The temperate phage lambda, which infects the bacterium Escherichia coli, belongs to Siphoviridae. The virion of the lambda phage comprises an icosahedral head and a long flexible tail. The tail, which comprises the tail tube and tail tip, connects with the head through the neck. The neck–tail complex comprises a channel formed by stacked 12-fold and hexameric rings and a 3-fold symmetrical tip.

Each of the 32 rings of gpV is assembled by 6 copies of the major tail protein gpV wrapped around an oligomer of the tape measure protein gpH. The 32 rings form a right-handed helix with an axial rise of approximately 42 Å and a twist of approximately 17.5° for 2 adjacent rings. GpV has 2 distinctive domains: the N-terminal domain (gpVN, residues 3–156) and the C-terminal domain (gpVC, residues 157–246). The inner tube structure could be reconstructed to a resolution of 3.5 Å, which enabled us to build an atomic model of the gpVN domain (S1B). The gpVN domain comprises a β-sandwich flanked by an α-helix. The β-sandwich is inserted by an E-loop (residues 50–78) between β3 and β4 and by an O-loop (residues 24–38) between β1 and β2. Six copies of the β-sandwich form the core of the tail tube ring. The outer surface of the ring is formed by the α-helix and O-loop. The inner surface of the gpV ring mostly bears a negative charge, similar to the tail tubes of phages T5 and 80α, facilitating DNA transfer. The architecture of gpVN is structurally conserved across the phage tails.

>MPVPNPTMPVKGAGTTLWVYKGSGDPYANPLSDVDWSRLAKVKDLTPGELTAESYDDSYLDDEDADWTATGQGQKSAGDTSFTLAWMPGEQGQQALLAWFNEGDTRAYKIRFPNGTVDVFRGWVSSIGKAVTAKEVITRTVKVTNVGRPSMAEDRSTVTAATGMTVTPASTSVVKGQSTTLTVAFQPEGVTDKSFRAVSADKTKATVSVSGMTITVNGVAAGKVNIPVVSGNGEFAAVAEITVTAS[12x]>MYEPKPEHRFTFGLWTVGNVGRDPFGDAVRERLDPVYVVHKLAELGAYGVNLHDEDLIPRGTPPQERDQIVRRFKKALDETGLKVPMVTANLFSDPAFKDGAFTSPDPWVRAYALRKSLETMDLGAELGAEIYVVWPGREGAEVEATGKARKVWDWVREALNFMAAYAEDQGYGYRFALEPKPNEPRGDIYFATVGSMLAFIHTLDRPERFGLNPEFAHETMAGLNFVHAVAQALDAGKLFHIDLNDQRMSRFDQDLRFGSENLKAAFFLVDLLESSGYQGPRHFDAHALRTEDEEGVWAFARGCMRTYLILKERAEAFREDPEVKELLAAYYQEDPAALALLGPYSREKAE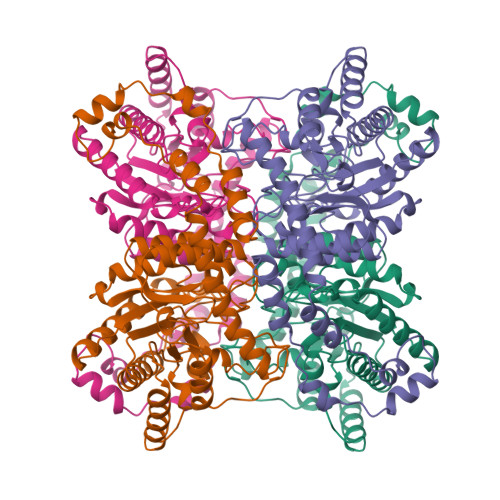ALKRAELPLEAKRRRGYALERLDQLAVEYLLGVRG[4x]> GGIAIYWGQNGNEGTLTQTCSTRKYSYVNIAFLNKFGNGQTPQINLAGHCNPAAGG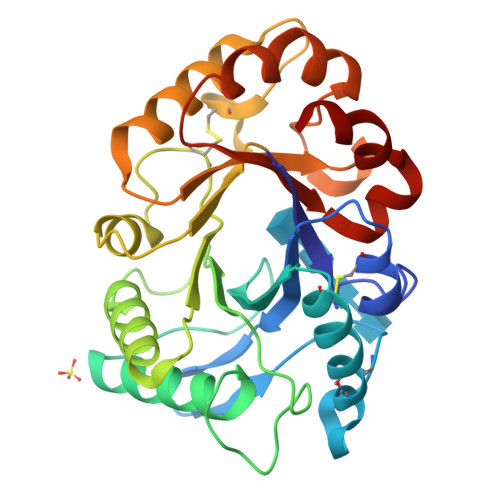CTIVSNGIRSCQIQGIKVMLSLGGGIGSYTLASQADAKNVADYLWNNFLGGKSSSRPLGDAVLDGIDFAIEHGSTLYWDDLARYLSAYSKQGKKVYLTAAPQCPFPDRYLGTALNTGLFDYVWVQFFNNPPCQYSSGNINNIINSWNRWTTSINAGKIFLGLPAAPEAAGSGYVPPDVLISRILPEIKKSPKYGGVMLWSKFYDDKNGYSSSILDSV>MARLDKSKVINSALELLNEVGIEGLTTRKLAQKLGVEQPTLYWHVKNKRALLDALAIEMHDRHQTHYLPLEGESWQDFLRNFAKSMRLALLSHRDGAKVSLGTRWTEQQYETAENMLAFLTQQGFSLENALYATDAVRVFTLGAVLLDQEQQVAKEERETPTPDSM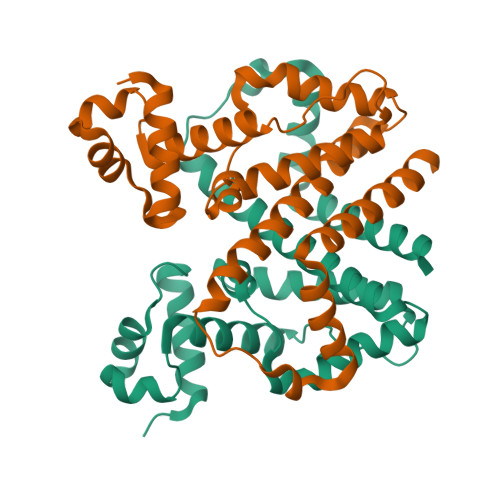PPLLRQAWELKVHQGAEPAFLFGLELIIAGLEKQLKRESGS[2x]> MSLQMVTVGHNIALIQPGFSLMNFDGQVFFFGQKGWPKRSCPTGVFHFDIKQNHLKLKPAIFSKDSCYLPPLRYPATCSYKGSIDSDKHQYIIHGGKTPNNELSDKIYIMSVACKNNKKVTFRCTEKDLVGDVPEPRYGHSIDVVYSRGKSMGVLFGGRSYMPS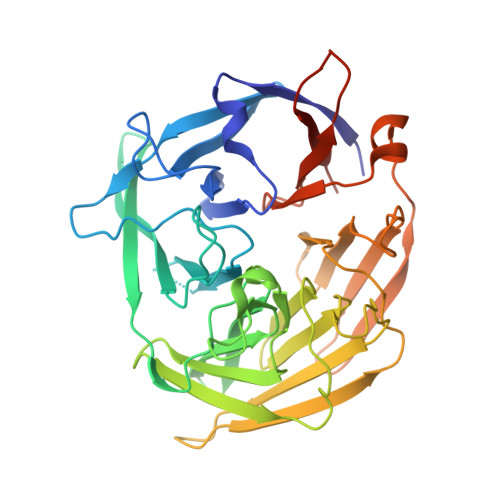TQRTTEKWNSVADCLPHVFLIDFEFGCATSYILPELQDGLSFHVSIARNDTVYILGGHSLASNIRPANLYRIRVDLPLGTPAVNCTVLPGGISVSSAILTQTNNDEFVIVGGYQLENQKRMVCSLVSLGDNTIEISEMETPDWTSDIKHSKIWFGSNMGNGTIFLGIPGDNKQAMSEAFYFYTLRCSEEDLSEDQ>SMNQLPRDVTHLLALVSSAIHAVENPFGANDLPYFRTLLKILFVVLRAAKQGTAKPGESNVAITQQVLTILDRVVARCFRALAALVHEQQQNATDGTTTAPEDLALITAILQACLSVPGIEQCQVQVLNIMAAHDVFQVAVALFSWADRLLPANPSPASSSTSTSATNPASGDPVYGELALLFLLELSALPALAEHLACDGLLGHLAAARLAGYMRRTNVGPFAENAGAARCYAIWAKCLLPLLLNILAALGSTVAPEVAWVLNQFPNLLQSSVERIEPPGFSRP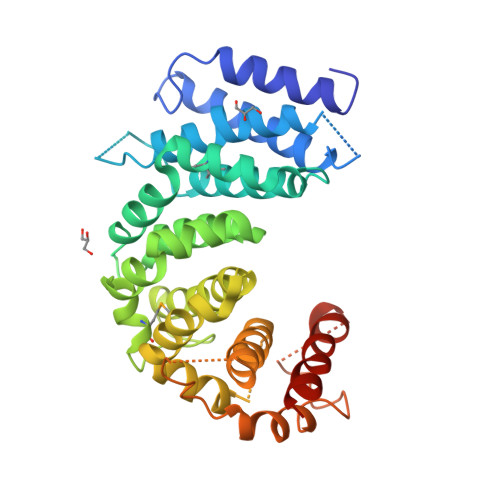TLSLASTPPRQKFISLLEISEIHSLALLTRVLAACRAQNARDVPEVTWDGAKVLECVEYWLRGRKVLRERLVPLGPREVEWRGMVATGGVVGVAGDGGEGCENRLEEKAVGLLVGVREVLEGGLEGEGE[8x]>[2x]EDPEVLAKNKGCVACHAIDTKMVGPAYKDVAAKFAG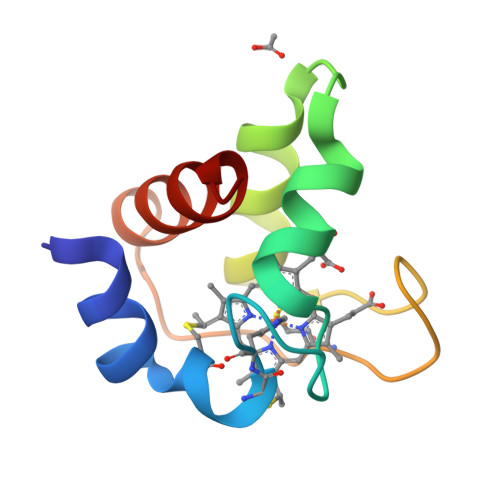QAGAEAELAQRIKNGSQGVWGPIPMPPNAVSDDEAQTLAKWVLSQK>GSHMTEAEYLANYDPKAFKAQLLTVDAVLFTYHDQQLKVLLVQRSNHPFLGLWGLPGGFIDETCDESLEQTVLRKLAEKTAVVPPYIEQLCTVGNNSRDARGWSVTVCYTALMSYQACQIQIASVSDVKWWPLADVLQMPLAFDHLQLIEQARERLTQKALYSLVPGFALSEPFTLPEL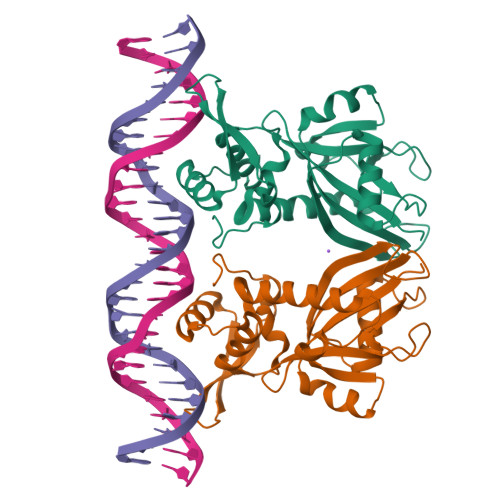QHVHEVLLGKPIQGKSFRRRVEQADLLIDTGLKRTERGRPANLYCLKPDTASYRFLRNLEC[2x]> SGSFELSVQDLNDLLSDGSGCYSLPSQPCNEVTPRI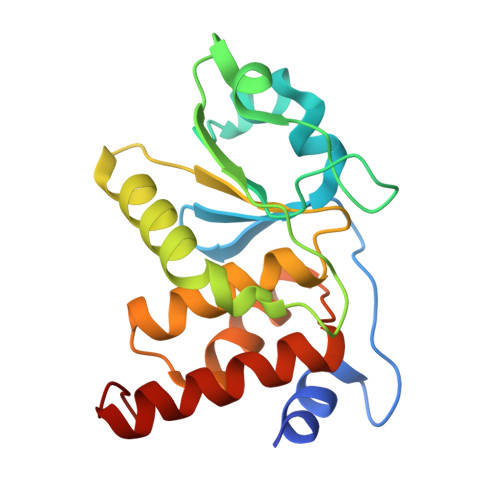YVGNASVAQDIPKLQKLGITHVLNAAEGRSFMHVNTNANFYKDSGITYLGIKANDTQEFNLSAYFERAADFIDQALAQKNGRVLVHSREGYSRSPTLVIAYLMMRQKMDVKSALSIVRQNREIGPNDGFLAQLCQLNDRLAKEGKLKP1,2,3,4-TETRAHYDROGEN-STAUROSPORINE | C28 H30 N4 O3 | 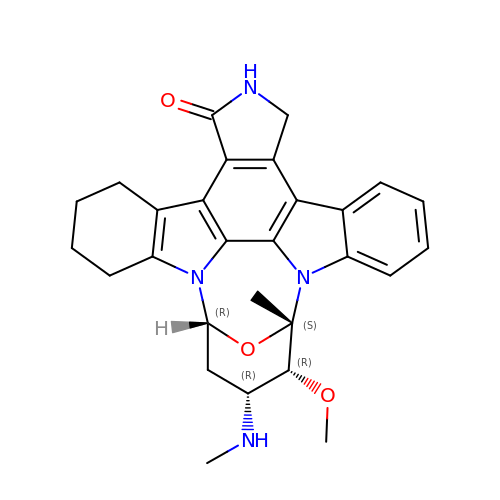KIZWKTROWIIMNN-FYTWVXJKSA-N>MGHHHHHHMSFEGKIVLVTGASRGIGRAIAETFVARGAKVIGTATSESGAEAISGYLGANGKGFMLNVKDAQSIDSVLASIRAEFGEIDILVNNAGITRDNLLMRMKDDEWEDILDTNLTSVFRLSKAVMCAMMKKRFGRIITIGSVVGTMGNAGQANYAAAKAGLIGFSKSLAREVASRGITVNVVAPGYIETDMTRALTDDQRAGILSSVPANRPGDAKEIASAVAFLASDEAGYITGETLHVNGGMYMI[2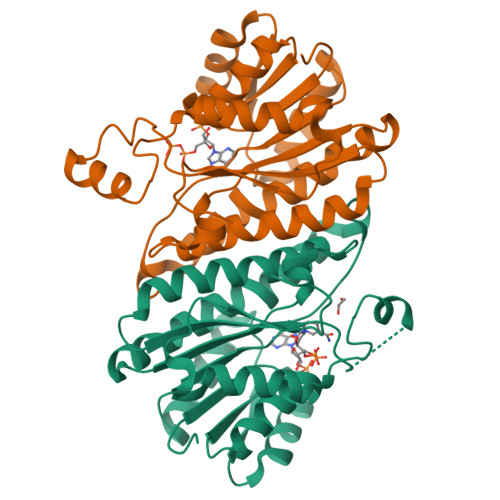x]> MSIKTTRDRVPTYQYNMNFEKLGKCIIINNKNFDKVTGMGVRNGTDKDAEALFKCFRSLGFDVIVYNDCSCAKMQDLLKKASEEDHTN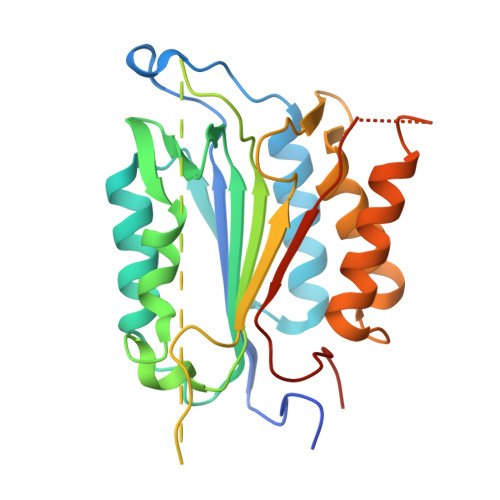AACFACILLSHGEENVIYGKDGVTPIKDLTAHFRGDRCKTLLEKPKLFFIQACRGTELDDGIQAASGPINDLVPRGSTDANPRYKIPVEADFLFAYSTVPGYYSWRSPGRGSWFVQALCSILEEHGKDLEIMQILTRVNDRVARHFESQSDDPHFHEKKQIPCVVSMLTKELYFSQLEHHHHHH N-[3'-cyano-4'-(2-methylpropyl)-2-(trifluoromethyl)biphenyl-4-yl]-2-[4-(ethylsulfonyl)phenyl]acetamide 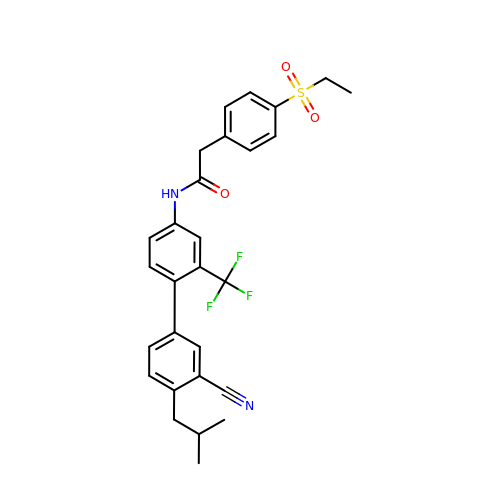| C28 H27 F3 N2 O3 S | IDDOTRDVQFMFJR-UHFFFAOYSA-N>[4x]KGPNLTEISKKITESNAVVLAVKEIETLLASIDELATKAIGKKIQQNGGLAVEAGHNGTLLAGAYTISKLITQKLDGLKNSEK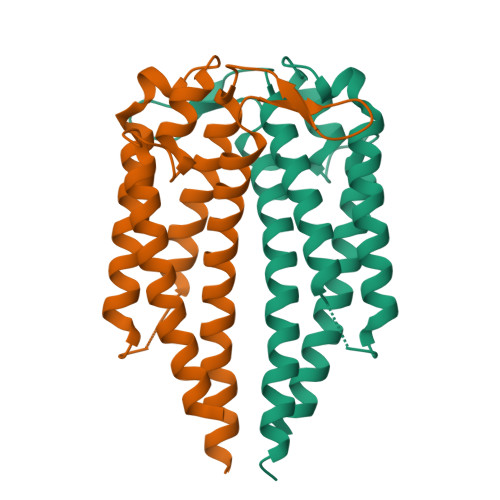LKEKIENAKKCSEDFTKKLEGEHAQLGIENVTDENAKKAILITDAAKDKGAAELEKLFKAVENLAKAAKEMLANSVKELTSP> MTTATAGLAVELKQSTAQAHEKAEHSTFMSDLLKGRLGVAEFTRLQEQAWLFYT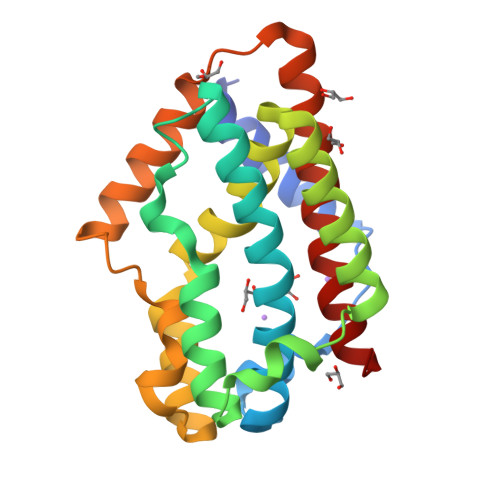ALEQAVDAVRASGFAESLLDPALNRAEVLARDLDKLNGSSEWRSRITASPAVIDYVNRLEEIRDNVDGPALVAHHYVRYLGDLSGGQVIARMMQRHYGVDPEALGFYHFEGIAKLKVYKDEYREKLNNLELSDEQREHLLKEATDAFVFNHQVFADLGKGL>MEKTEKSGLSDSKKLSVLLTGFEPFGGEKVNPSMRIVKRLSKAVFPHISLHTLILPVSYQKSTEVLEEYYKTNNIDIALHLGQAGGSAGIRLERVAINLLDSKHPDNDGQVKEDVSIIDNGPDAYMTRVKIKAVAELLKKKKIPAFVSYTAGQYICNEVYYYSLHRS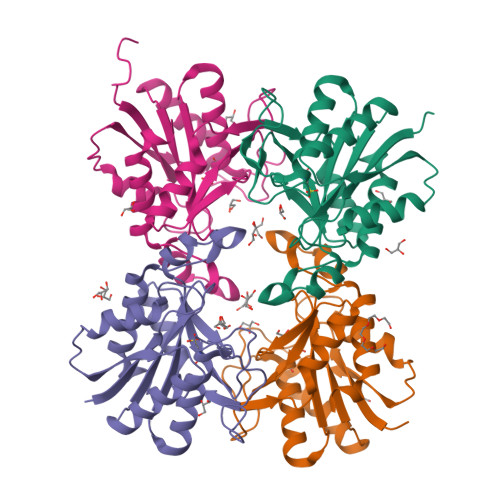NVTGTPKHALFVHLPFLPEQVATKEGKLEKLPSMTLELQTKAVRLILENLKEFI[4x]1-[5-[4-fluoranyl-2-[2-(1,3,5-trimethylpyrazol-4-yl)ethoxy]phenyl]-2~{H}-indazol-3-yl]-~{N},~{N}-dimethyl-methanamine | C24 H28 F N5 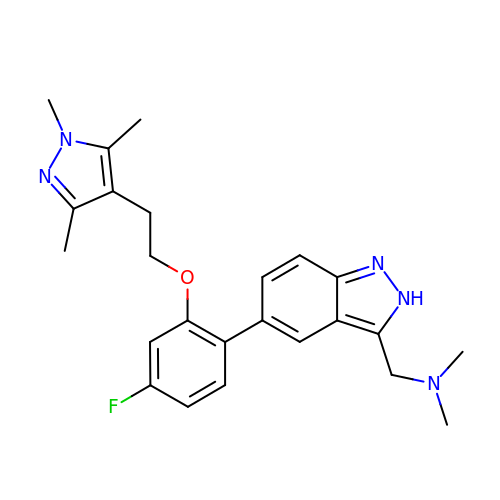O | CGEINWMYWNHNPM-UHFFFAOYSA-N>MTDMNILDLFLKASLLVKLIMLILIGFSIASWAIIIQRTRILNAAAREAEAFEDKFWSGIELSRLYQESQGKRDNLTGSEQIFYSGFKEFVRLHRANSHAPEAVVEGASRAMRISMNRELENLETHIPFLGTVGSISPYIGLFGTVWGIMHAFIALGAVKQATLQMVAPGIAEALIATAIGLFAAIPAVMAYNRLNQRVNKLELNYDNFMEEFTAILHRQAFTVSESNKG[5x];>[2x]MARARGRGRRDLKSEINIVPLLDVLLVLLLIFMATAPIITQSVEVDLPDATESQAVSSNDNPPVIVEVSGIGQYTVVVEKDRLERLPPEQVVAEVSSRFKANPKTVFLIGGAKDVPYDEIIKALNLLHSAGVKSVGLMTQPI

The Tol-Pal system is essential for maintaining outer membrane (OM) stability during cell division in Gram-negative bacteria. The inner membrane complex TolQRA harnesses proton motive force (PMF) to establish transient interactions within the periplasm, thereby coordinating cell envelope remodeling and facilitating OM invagination at division sites. TolQ forms a pentameric structure similar to that of MotA and ExbB, exhibiting a volcano-like configuration with a narrow periplasmic end and a wider cytoplasmic base. The pentameric TolQ encapsulates the dimeric TolR through its N-terminal transmembrane helices at the periplasmic end.

To explore the dynamic motion of the TolQRA complex, we aimed to capture its distinct states using styrene-maleic acid (SMA) polymers. Two distinct structural classes with high resolutions were determined at 2.92 and 3.28 Å, respectively, with one class lacking density for TolA (hereafter TolQ5R2) and the other displaying density corresponding to one copy of TolA (hereafter TolQ5R2A). The TolA molecule bound in TolQ5R2A is positioned consistently with its location on the TolQ1 subunit in the nanodisc TolQ5R2A3 structure. The superimposition of the TolQ5R2 and TolQ5R2A structures onto the TolQ5R2A3 structure shows root-mean-square deviation (RMSD) values of 1.31 and 2.52 Å, respectively, based on the alignment of 217 Cα atoms. The superimposition of these structures, utilizing the TolR dimer as a reference, revealed that the TolQ5R2 structure slightly rotated compared to TolQ5R2A3. The morphing transition between TolQ5R2A3 and TolQ5R2 demonstrates a prominent shutter-like rotation in the cytoplasmic termini of TolQ in relation to the central TolR dimer. When viewed from the cytoplasmic side of the pentamer, TolQ5R2A3 features an oval-shaped cytoplasmic opening, TolQ5R2 presents a round opening, and TolQ5R2A displays a split between TolQ1 and TolQ5 as well as between TolQ3 and TolQ4. Conformational variation primarily arises from the cytoplasmic half of the TM2 helix, which contains three arginine residues (R110, R113, and R118). These residues form salt bridges with glutamic acid residues (E211 or E212) and hydrogen bonds with H218 in TM3 of adjacent TolQ subunits. To investigate how D23 protonation in TolR influences conformational dynamics during TolQRA rotation, we performed MD simulations on different protonation states of the SMA-captured intermediate TolQ5R2 structure. Protonation of D23 in both TolR(A) and TolR(B) enhanced structural stability, as reflected by consistent TolR_D23–TolQ_T178 distances in the simulations.> ELTPDQQTLLHFIMDSYNKQRMPQEITNKILKEEFSAEENFLILTEMATNHVQVLV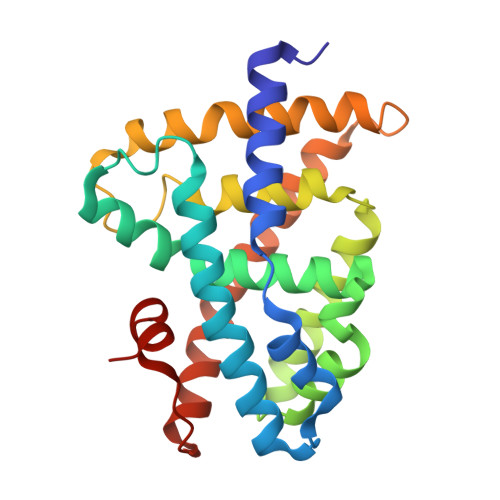EFTKKLPGFQTLDHEDQIALLKGSAVEAMFLRSAEIFNKKLPSGHSDLLEERIRNSGISDEYITPMFSFYKSIGELKMTQEEYALLTAIVILSPDRQYIKDREAVEKLQEPLLDVLQKLCKIHQPENPQHFAELLGRLTELRTFNHHHAEMLMSWRVNDHKFTPLLEEIWDVQ>[6x]MAKSTTFFISLTLPFLLLSVVTATYYQSMSPTVLGFQEEKFTHLHFYFHDVVTGPKPSMVIVAEPNGKA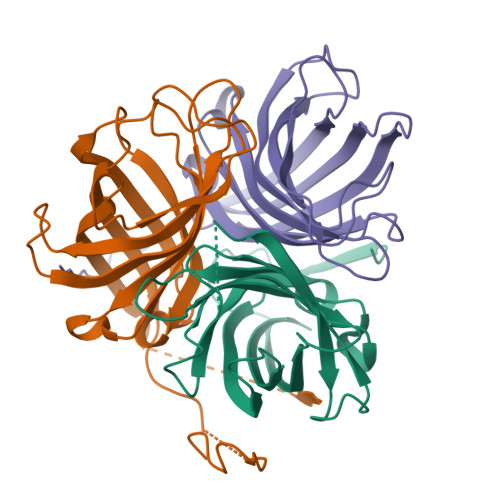KNSLPFGTVVAMDDPLTVGPESDSKLVGKAQGIYTSISQEEMGLMMVMTMAFSDGEFNGSTLSILARNMIMSEPVREMAIVGGTGAFRFARGYAQAKFYSVDFTKGDAIVEYDIFVFHYKGELNSKLEGKPIPNPLLGLDSTRTGHHHHHH> MKLKKIVFTLIALGLFSCKTTSVLVKNEPQLKTPKNVILLISDGAGLSQISSTFYFKEGTPNYTQFKNIGLIKTSSSREDVTDSASGATAFSCGIKTYNAAIGVADDSTAVKSIVEIAALNNIKTGVVATSSITHATPASFYAHALNRGLEEEIAMDMTESDLDFFAGGGLNYFTSRKDKKDVLAILKGNQFTINTTGLTDFSSIASNRKMGFLLADEAMPTMESGRGNFLSAATDLAIQFLSKD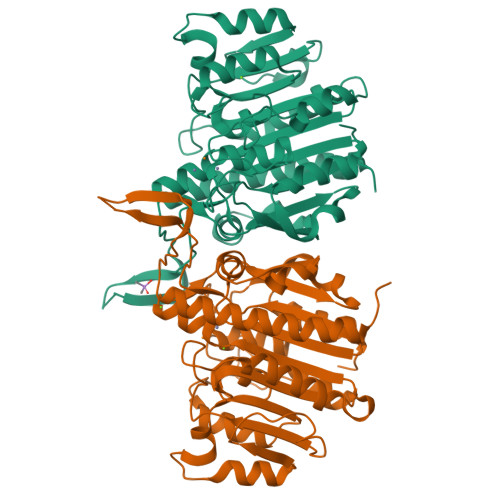NSAFFIMSEGSQIDWGGHANNASYLISEINDFDDAIGTALAFAKKDGNTLVIVTSDHETGGFTLAAKKNKREDGSEYSDYTSIGPSFSTGGHSATLIPVFAYGPGSEEFIGIYENNEIFHKILKVTKWNQ;> MKLKKIVFTLIALGLFSCKTTSVLVKNEPQLKTPKNVILLISDGAGLSQISSTFYFKSGTPNYTQFKNIGLIKTSSSREDVTDSASGATAFSCGIKTYNAAIGVADDSTAVKSIVEIAALNSIKTGVVATSSITHATPASFYAHALNRGLEEEIAMDMTESDLDFFAGGGLNYFTSRSDSKDVLAILKGNQFTINTTGLTDFSSIASNRKMGFLLADEAMPTMEKGRGNFLSAATDLAIQFLSKDNSAFFIMSEGSQIDWGGHANNASYLISEINDFDDAIGTALAFAKSDGNTLVIVTSDHETGGFTLAAKSNKREDGSEYSDYTEIGPTFSTGGHSATLIPVFAYGPGSEEFIGIYENNEIFHKILKVTKWNQ>GPMGKPARKGCEWKRFLKNNWVLLSTVAAVVLGITTGVLVREHSNLSTLEKFYFAFPGEILMRMLKLIILPLIISSMITGVAALDSNVSGKIGLRAVVYYFCTTLIAVILGIVLVVSIKPGVTQKVGEIARTGSTPEVSTVDAM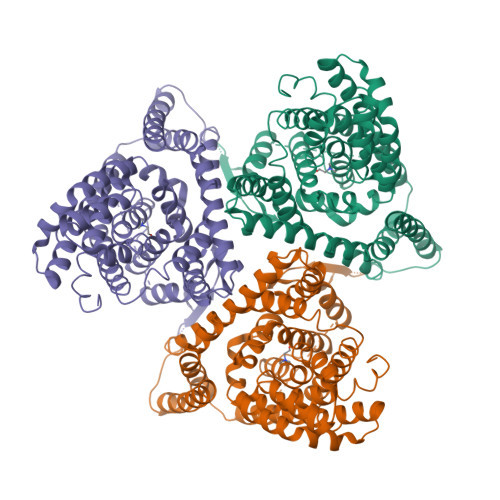LDLIRNMFPENLVQACFQQYKTKREEVKPPSDPEMNMTEESFTAVMTTAISKNKTKEYKIVGMYSDGINVLGLIVFCLVFGLVIGKMGEKGQILVDFFNALSDATMKIVQIIMCYMPLGILFLIAGKIIEVEDWEIFRKLGLYMATVLTGLAIHSIVILPLIYFIVVRKNPFRFAMGMAQALLTALMISSSSATLPVTFRCAEENNQVDKRITRFVLPVGATINMDGTALYEAVAAVFIAQLNDLDLGIGQIITISITATSASIGAAGVPQAGLVTMVIVLSAVGLPAEDVTLIIAVDWLLDRFRTMVNVLGDAFGTGIVEKLSKKELEQMDVSSEVNIVNPFALESTILDNEDSDTKKSYVNGGFAVDKSDTISFTQTSQF[3x]> GHMENFRKVRSEEAPAGCGAEGGGPGSGPFADLAPGAVHMRV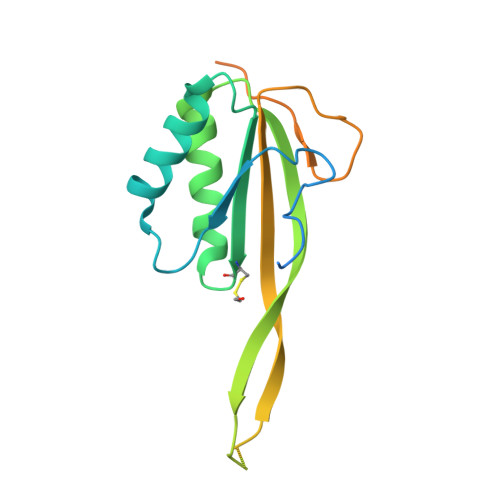KEGSKIRNLMAFATASMAQPATRAIVFSGCGRATTKTVTCAEILKRRLAGLHQVTRLRYRSVREVWQSLPPGPTQGQTPGEPAASLSVLKNVPGLAILLSKDALDPRQPGYQPPNPHPGPSSPPAAPASKRSLGEPAAGEGSAKRSQPEPGVADEDQTA> TENILRKSDEEIQKEITARVKALESMLIEQGILTTSMIDRMAEIYENEVGPHLGAKVVVKAWTDPEFKKRLLADGTEACKELGIGGLQGEDMMWVENTDEVHHVVVCSLCSCYPWPVLGLPPNWFKEPQYRSRVVREPRQLLKEEFGFEVPPSKEIKVWDSSSEMRFVVLPQRPAGTDGWSEEELATLVTRE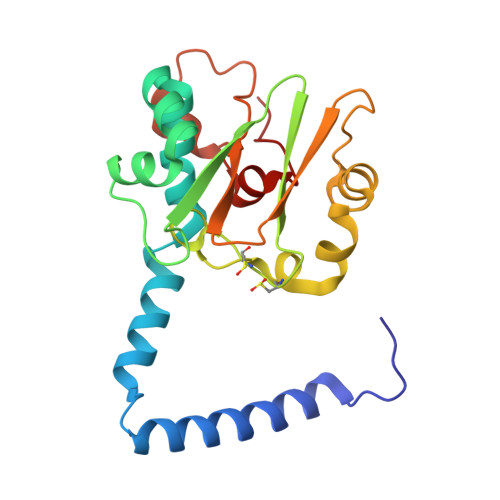SMIGVEPAKAV>MAKPCGVRLSGEARKQVDVFRQNLFQEADDFLCTFLPRKIISLSQLLQEDSLNVADLSSLRAPLDIPIPDPPPKDDEMETDKQEKKEVPKCGYLPGNEKLLALLALVKPEVWTLKEKCILVITWIQHLIPKIED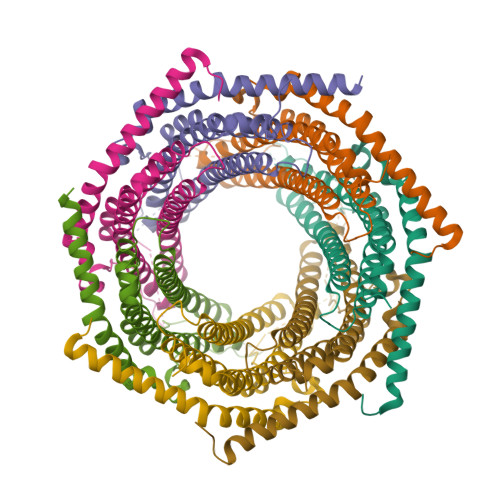GNDFGVAIQEKVLERVNAVKTKVEAFQTTISKYFSERGDAVAKASKDTHVMDYRALVHERDEAAYGALRAMVLDLRAFYAELYHIISSNLEKIVNPKGEEKPSMY[7x]> IVGGYE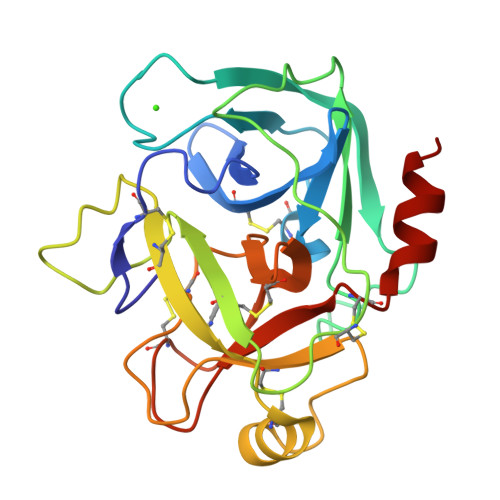CKAYSQPHQVSLNSGYHFCGGSLVNENWVVSAAHCYKTRVEVRLGEHNIKVTEGSEQFISSSRVIRHPNYSSYNIDNDIMLIKLSKPATLNTYVQPVALPSSCAPAGTMCTVSGWGNTMSSTADKNKLQCLNIPILSYSDCNNSYPGMITNAMFCAGYLEGGKDSCQGDSGGPVVCNGELQGVVSWGYGCAEPGNPGVYAKVCIFNNWLTSTMATY>SAEEELKKLLEENIKLIEELLEEVKHNDPELLLSVLEVLVRSVHVIAEVAREQGNEELLERAARLAEEAAYQAEEVAREARKRGNLELALKALQILVNAAYVLAEIARDRGNEELLQKAHELAREALRQVKEILEQARKEGNLELVIIALRLHTEIMRVLVEI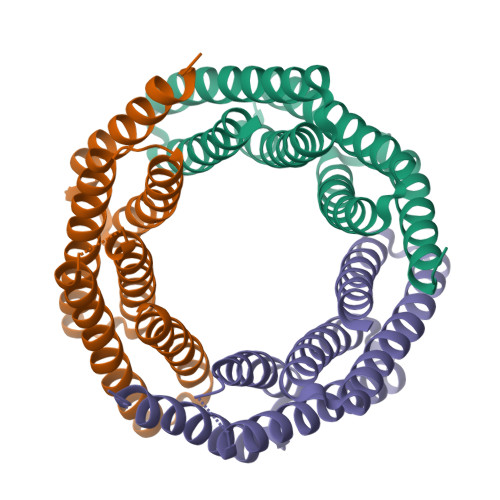WRHR[3x]> MTQFTQNTAMPSSLWQYWRGLSGWNFYFLVKFGLLWAGYLNFHPLLNLVFAAFLLMPLPRYSLHRLRHWIALPIGFALFWHDTWLPGPESIMSQGSQVAGFSTDYLIDLVTRFINWQMIGAIFVLLVAWLFLSQWIRITVFVVA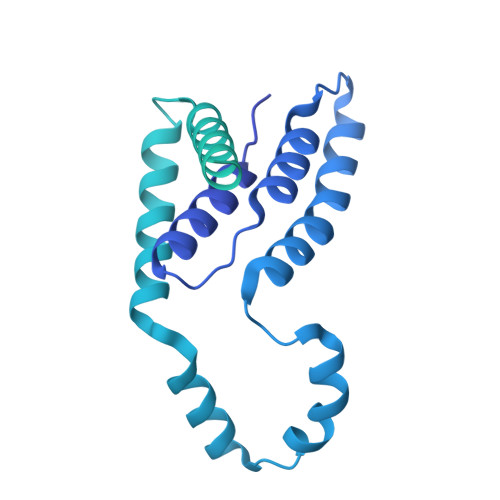ILLWLNVLTLAGPSFSLWPAGQPTTTVTTTGGNAAATVAATGGAPVVGDMPAQTAPPTTANLNAWLNNFYNAEAKRKSTFPSSLPADAQPFELLVINICSLSWSDIEAAGLMSHPLWSHFDIEFKNFNSATSYSGPAAIRLLRASCGQTSHTNLYQPANNDCYLFDNLSKLGFTQHLMMGHNGQFGGFLKEVRENGGMQSELMDQTNLPVILLGFDGSPVYDDTAVLNRWLDVTEKDKNSRSATFYNTLPLHDGNHYPGVSKTADYKARAQKFFDELDAFFTELEKSGRKVMVVVVPEHGGALKGDRMQVSGLRDIPSPSITDVPVGVKFFGMKAPHQGAPIVIEQPSSFLAISDLVVRVLDGKIFTEDNVDWKKLTSGLPQTAPVSENSNAVVIQYQDKPYVRLNGGDWVPYPQDYKDDDDK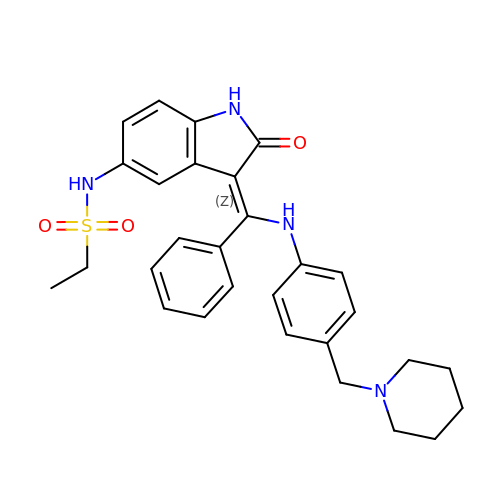N-{(3Z)-2-oxo-3-[phenyl({4-[(piperidin-1-yl)methyl]phenyl}amino)methylidene]-2,3-dihydro-1H-indol-5-yl}ethanesulfonamide | C29 H32 N4 O3 S | GLDSKRNGVVYJAB-DQSJHHFOSA-N>GSFTSSGSDSQLLLEPGDRSHWCVVAYWEEKTRVGRLYCVQEPSLDIFYDLPQGNGFCLGQLNSDNKSQLVQKVRSKIGCGIQLTREVDGVWVYNRSSYPIFIKSATLDNPDSRTLLVHKVFPGFSIKAFDYEKAYSLQRPNDHEFMQQPWTGFTV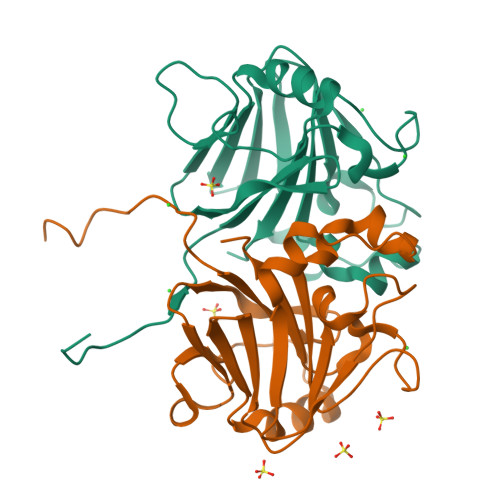QISFVKGWGQCYTRQFISSCPCWLEVIFNSR[4x]>[8x]MKFLVNVALVFMVVYISYIYADYKDDDDKLVPRGGGSIINETADDIVYRLTVIIDDRY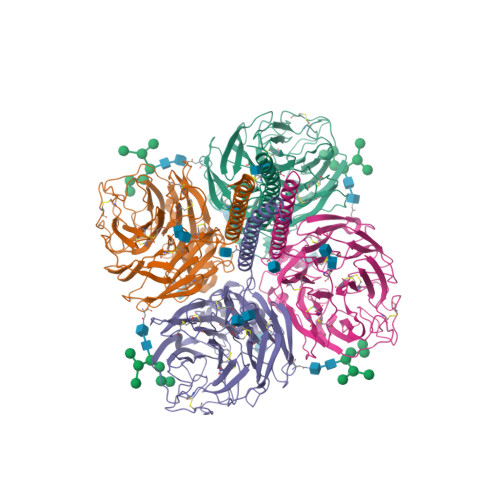ESLKNLITLRADRLEMIINDNVSTILARDFNNLTKGLCTINSWHIYGKDNAVRIGEDSDVLVTREPYVSCDPDECRFYALSQGTTIRGKHSNGTIHDRSQYRALISWPLSSPPTVYNSRVECIGWSSTSCHDGKTRMSICISGPNNNASAVIWYNRRPVTEINTWARNILRTQESECVCHNGVCPVVFTDGSATGPAETRIYYFKEGKILKWEPLAGTAKHIEECSCYGERAEITCTCRDNWQGSNRPVIRIDPVAMTHTSQYICSPVLTDNPRPNDPTVGKCNDPYPGNNNNGVKGFSYLDGVNTWLGRTISIASRSGYEMLKVPNALTDDKSKPTQGQTIVLNTDWSGYSGSFMDYWAEGECYRACFYVELIRGRPKEDKVWWTSNSIVSMCSSTEFLGQWDWPDGAKIEYFL(3S)-3-(1H-indol-3-ylmethyl)-3,4-dihydro-1H-1,4-benzodiazepine-2,5-dione 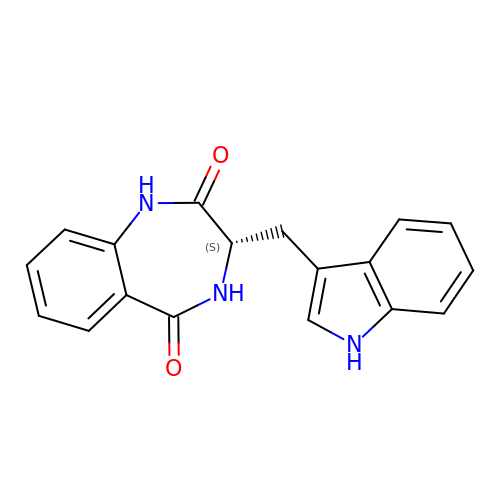| C18 H15 N3 O2 | AQDZAHJUWYRHGM-INIZCTEOSA-N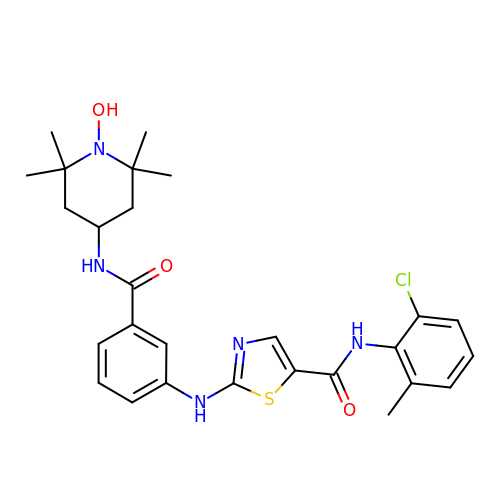~{N}-(2-chloranyl-6-methyl-phenyl)-2-[[3-[(2,2,6,6-tetramethyl-1-oxidanyl-piperidin-4-yl)carbamoyl]phenyl]amino]-1,3-thiazole-5-carboxamide | C27 H32 Cl N5 O3 S | NBHNLUWASSBGER-UHFFFAOYSA-N> GPTVVDQIRLWQLELDRVITYEGSLYS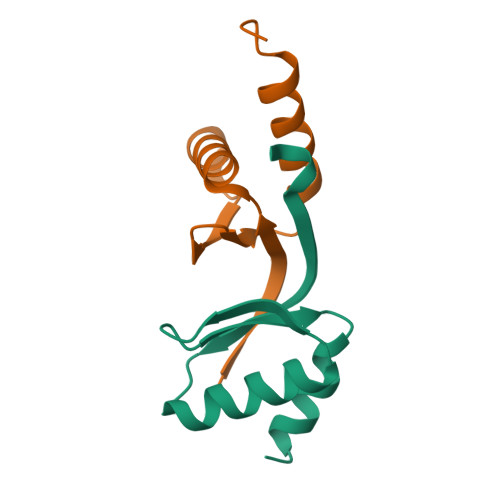DFETSQEYNLLSKYAQDIGVLLWKDDKKKKFFISKEGNSQVLDFAKRKLKKKQ;> ARARKGALVQCDPSIKALILQIDAKMSDIVLEELDDTHLLVNPSKVEFVKHELNRLLSKNIYNPMDEEENQ Conjugative type IV secretion systems (T4SS) mediate bacterial conjugation, a process that enables the unidirectional exchange of genetic materials between a donor and a recipient bacterial cell. Bacterial conjugation is the primary means by which antibiotic resistance genes spread among bacterial populations. The recent cryo-electron microscopy (cryo-EM) structure of the conjugative Type 4 Secretion System (T4SS) encoded by the plasmid R388 revealed that the remaining VirB proteins form a large assembly organised into four sub-complexes: the outer membrane core complex (OMCC), the stalk, the arches and the inner membrane complex (IMC). Previously, we solved the cryo-electron microscopy (cryo-EM) structure of a conjugative T4SS. In this article, based on additional data, we present a more complete T4SS cryo-EM structure than that published earlier.

The Stalk is 5-fold symmetrical and is made of TrwJ/VirB5 and TrwI/VirB6, with TrwI/VirB6 embedded into the IM and hypothesised to serve as a platform for pilus subunit recruitment and assembly. Indeed, TrwI/VirB6 features two key sites: a VirB2-binding site at its base in the IM, and a pilus-assembly site at its top. TrwJ/VirB5 is located at the tip of the stalk, and is expected to be recruited at the pilus tip during the early step of pilus biogenesis. In these regions of the T4SS structure, improved resolution resulted in better-defined densities at the tip of TrwJ/VirB5. In the TrwJ/VirB5 N-terminal tip, 11 residues could be added at the N-terminus (residues Gln23-Ala33). Gln23 is the very N-terminal residue in the protein after signal sequence cleavage. Middle panel, this newly built region is hydrophobic in nature. Viewed from the top, the hydrophobic tip of TrwJ/VirB5 resembles a needle (insets of each panel).

>[5x]MKKLVMTAAVAAILGAASPVMAQGIPVFDGTRALDFVQQFARMKEQLDTAKDQLAEAQRMYEAVTGGRGLGDLMRNAQLREYLPDDLRTVYDSANGGGYSGISGSINDILRDERLNGSVADMRRSIEERSRTAAATDKAVGLRAYEGAQQRLAQIEGLMDEISRTQDQKAIEELQARIAGEQAAIQNETTKLQMIAQLRQAEQALISEQRRERNMRILSSGNQGMPTIQ;>MAFELFTPLFNKIDQTTATYVTDISSRAIAAITPVVSVGLTLGFITYGWLIIRGAVEMPVAEFLNRCLRIGIIVSIALAGGLYQGEIANAITTVPDELASALLGNPTQGASAAALVDQSAQQGFDRASEAFEEAGFFSSDGLLYGLFGIIILLATGLLAAIGGAFLLLAKIALALLAGLGPLFILALIWQPTHRFFDQWAQQVLNYGLLIVLFAAVFGLLMQIFGSYMADLRFDGAQNVAYAIGGSVILSIVSIVLLMQLPSIASGLAGGIGLGYMWELRSMRSGAGAAMRGGRAMARGARAAPGAARGAAVGAANMAKTVATGGAGVARAAAGYFRGRKAG[5x]>[12x]MERFLLNSTVLLYRLSTVSLDEVSLDERVESSVFLAQYEQARSLPDHVAKSAWSYLVQQIKQRNMKLGPVAILRLIAEKFIKNEKGGPKIDLPMFSEWQTLMSRVSCLPIIACHQVFNPGPASQEYSFRWPLYPYHPTVEDYITRECLHETHQHLNGSTSAEECWLDALKHPEACLRDFEKGWASQEMKQLCAQIDPSLTPRIFKDRLQIACNIREILCRVAQGVELPEWIASMQNPQQLANSTILHNGREYGFATVWPIDDKYSQESEFCWLTGLLEKWRFNAPEGLERLLWIYLLIQNQYLTLLVQRDDFFGFEQFQNYTMTELREETEKSYLSRFKHAHGAGVYSQVRYLEGRFAPKSDPNKMQKLLFSVLRGYWEYLSAHMSMEWVHEKPLTISQVLDNLELVEPHGKCVELALVPHFIKRKPKNGEAYPHALLFKDLKNQAAILMDMLKSEPRLTGWIRGVDAAANEMHAP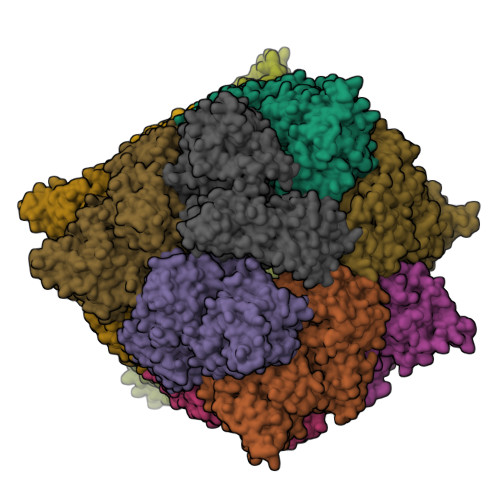PELFCPLFRVLAKSGIAHFTYHVGEDFPHLISGIRSIDDALRFLPLRNGDRLGHCTAIGITPSIWKRSLPLSLSMTKETRLLDLVFIWRELRSHPELLRYASDAAIEAVRLAHKVFSLEEEVSITTLDQVFEMRGLLAESEGLLSELNEPLKPKSLWLEEYERARELVKTTGMKRPLKLYKQWLTSDNVRKQRAEYVEVALEYLPDEAVVALQQAVMAKMADRNIAIECPPTSNTRISQYRNVSEHHIFRWMGLPGEAIEGDVPMSICLGSDDPGIFAADLKSEFYHLFVVLTRKFGLSPADALRKVAEVNENGRIYRFHDV>[4x]MPKRTDIKSILILGAGPIVIGQACEFDYSGAQACKALREEGYRVILVNSNPATIMTDPEMADATYIEPIHWEVVRKIIEKERPDAVLPTMGGQTALNCALELERQGVLEEFGVTMIGATADAIDKAEDRRRFDVAMKKIGLETARSGIAHTMEEALAVAADVGFPCIIRPSF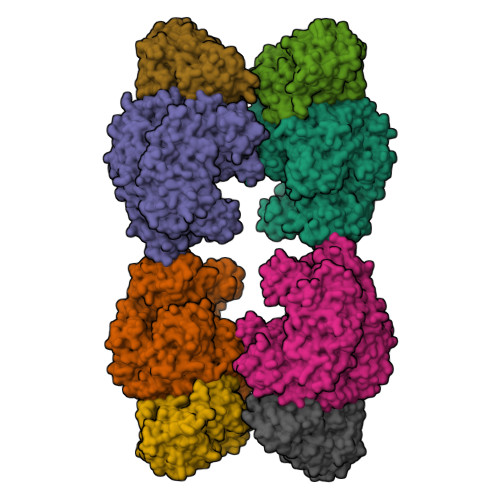TMGGSGGGIAYNREEFEEICARGLDLSPTKELLIDESLIGWKEYEMEVVRDKNDNCIIVCSIENFDAMGIHTGDSITVAPAQTLTDKEYQIMRNASMAVLREIGVETGGSNVQFAVNPKNGRLIVIEMNPRVSRSSALASKATGFPIAKVAAKLAVGYTLDELMNDITGGRTPASFEPSIDYVVTKIPRFNFEKFAGANDRLTTQMKSVGEVMAIGRTQQESLQKALRGLEVGATGFDPKVSLDDPEALTKIRRELKDAGADRIWYIADAFRAGLSVDGVFNLTNIDRWFLVQIEELVRLEEKVAEVGITGLNADFLRQLKRKGFADARLAKLAGVREAEIRKLRDQYDLHPVYKRVDTCAAEFATDTAYMYSTYEEECEANPSTDREKIMVLGGGPNRIGQGIEFDYCCVHASLALREDGYETIMVNCNPETVSTDYDTSDRLYFEPVTLEDVLEIVRIEKPKGVIVQYGGQTPLKLARALEAAGVPVIGTSPDAIDRAEDRERFQHAVERLKLKQPANATVTAIEMAVEKAKEIGYPLVVRPSYVLGGRAMEIVYDEADLRRYFQTAVSVSNDAPVLLDHFLDDAVEVDVDAICDGEMVLIGGIMEHIEQAGVHSGDSACSLPAYTLSQEIQDVMRQQVQKLAFELQVRGLMNVQFAVKNNEVYLIEVNPRAARTVPFVSKATGVPLAKVAARVMAGKSLAEQGVTKEVIPPYYSVKEVVLPFNKFPGVDPLLGPEMRSTGEVMGVGRTFAEAFAKAQLGSNSTMKKHGRALLSVREGDKERVVDLAAKLLKQGFELDATHGTAIVLGEAGINPRLVNKVHEGRPHIQDRIKNGEYTYIINTTSGRRAIEDSRVIRRSALQYKVHYDTTLNGGFATAMALNADATEKVISVQEMHAQIK;>MIKSALLVLEDGTQFHGRAIGATGSAVGEVVFNTSMTGYQEILTDPSYSRQIVTLTYPHIGNVGTNDADEESSQVHAQGLVIRDLPLIASNFRNTEDLSSYLKRHNIVAIADIDTRKLTRLLREKGAQNGCIIAGDNPDAALALEKARAFPGLNGMDLAKEVTTAEAYSWTQGSWTLTGGLPQAKKEDELPFHVVAYDFGAKRNILRMLVDRGCRLTIVPAQTSAEDVLKMNPDGIFLSNGPGDPAPCDYAITAIQKFLETDIPVFGICLGHQLLALASGAKTVKMKFGHHGGNHPVKDVEKNVVMITAQNHGFAVDEATLPANLRVTHKSLFDGTLQGIHRTDKPAFSFQGHPEASPGPHDAAPLFDHFIELIEQYRKTAK[4x]>MRINHNIAALNTLNRLSSNNSASQKNMEKLSSGLRINRVGDDAAGLAISEKMRGQIRGLEMASKNSQDGISLIQTAEGALTETHAILQRVRELVVQAGNTGTQ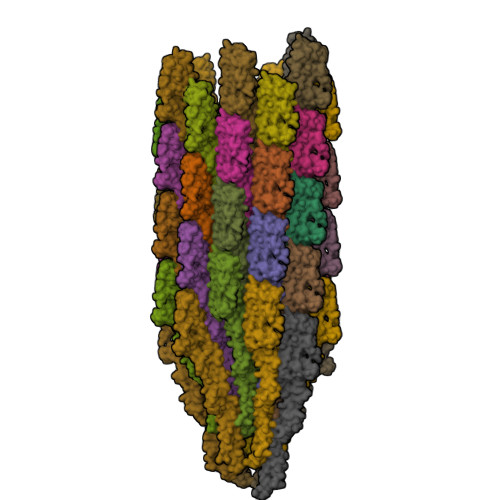DKATDLQSIQDEISALTDEIDGISNRTEFHGKKLLDGTYKVDTATPANQKNLVFQIGANATQQISVNIEDMGADALGIKEADGSIAALHSVNDLDVTKFADNAADCADIGFDAQLKVVDEAINQVSSQRAKLGAVQNRLEHTINNLSASGENLTAAESRIRDVDMAKEMSEFTKNNILSQASQAMLAQANQQPQNVLQLLR[46x]>GMNGEAICSALPTIPYHKLADLRYLSRGASGTVSSARHADWRVQVAVKHLHIHTPLLDSERKDVLREAEILHKARFSYILP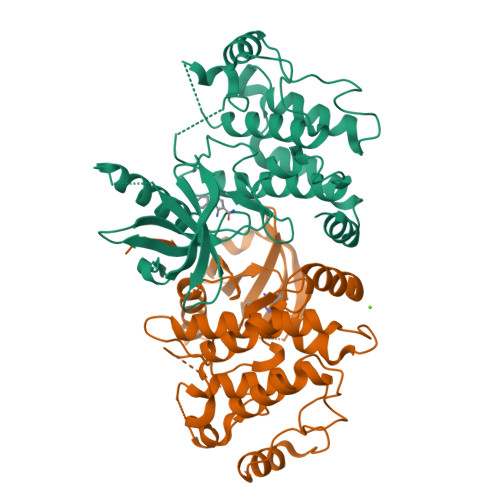ILGICNEPEFLGIVTEYMPNGSLNELLHRKTEYPDVAWPLRFRILHEIALGVNYLHNMTPPLLHHDLKTQNILLDNEFHVKIADFGLSKWRMMSLSQSRSSKSAPEGGTIIYMPPENYEPGQKSRASIKHDIYSYAVITWEVLSRKQPFEDVTNPLQIMYSVSQGHRPVINEESLPYDIPHRARMISLIESGWAQNPDERPSFLKCLIELEPVLRTFEEITFLEAVIQLK[2x]>GPMGWPPG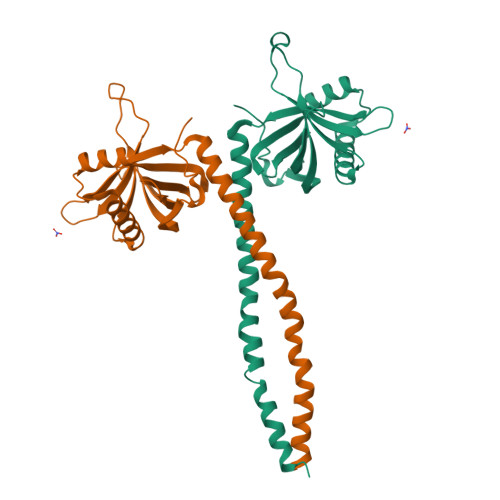SEDSYSAKMDYGKSVVNILPSVEMLVNFNGDMTRSSKRSCLLYAERVDFKELLQLRLTEKSDQRRMYITTVDSASFQDLKQDQSLNVSFSGFIDNVVRMLKDCQSGKLELHLTTRDQNLSSGREVHDYYLQFVEIRSDKNLVHLSLPCRSAPLNTVLFYINSMLEASHKKQYILEQSMQQMQAEINAQRAHAERLTTENTNLREALAENTR[2x]>[4x]MASRGSHHHHHHGAGDRGPEFELGTRGSMNVYQLKEELIEYAKSIGVDKIGFTTADTFDSLKDRLILQESLGYLSGFEEPDIEKRVTPKLLLPKAKSIVAIALAYPSRMKDAPRSTRTERRGIFCRASWGKDYHDVLREKLDLLEDFLKSKHEDIRTKSMVDTGELSDRAVAERAGIGFSAKNCMITTP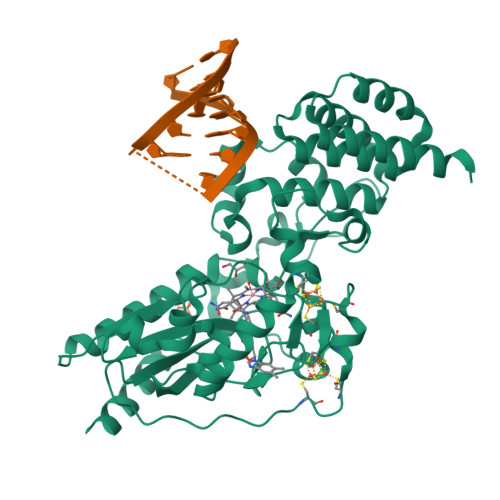EYGSYVYLAEMITNIPFEPDVPIEDMCGSCTKCLDACPTGALVNPGQLNAQRCISFLTQTKGFLPDEFRTKIGNRLYGCDTCQTVCPLNKGKDFHLHPEMEPDPEIAKPLLKPLLAISNREFKEKFGHVSGSWRGKKPIQRNAILALAHFKDASALPELTELMHKDPRPVIRGTAAWAIGKIGDPAYAEELEKALEKEKDEEAKLEIEKGIELLKASGMTKQGLSGSLEVDLQGDHGLSAWSHPQFEK>[2x]TEKKYIVALDQGTTSSRAVVMDHDANIISVSQREFEQIYPKPGWVEHDPMEIWATQS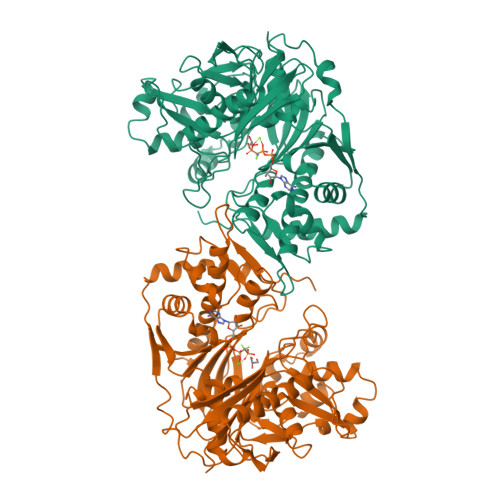WTLVEVLAKADISSDQIAAIGITNQRETTIVWEKETGKPIYNAIVWQCRRTAEICEHLKRDGLEDYIRSNTGLVIDPYFSGTKVKWILDHVEGSRERARRGELLFGTVDTWLIWKMTQGRVHVTDYTNASRTMLFNIHTLDWDDKMLEVLDIPREMLPEVRRSSEVYGQTNIGGKGGTRIPISGIAGDQQAALFGQLCVKEGMAKNTYGTGCFMLMNTGEKAVKSENGLLTTIACGPTGEVNYALEGAVFMAGASIQWLRDEMKLINDAYDSEYFATKVQNTNGVYVVPAFTGLGAPYWDPYARGAIFGLTRGVNANHIIRATLESIAYQTRDVLEAMQADSGIRLHALRVDGGAVANNFLMQFQSDILGTRVERPEVREVTALGAAYLAGLAVGFWQNLDELQEKAVIEREFRPGIETTERNYRYAGWKKAVKRAMAWEEHDE>[2x]MISVTDLRPGTKVKMDGGLWECVEYQHQKLGRGGAKVVAKFKNLETGATVE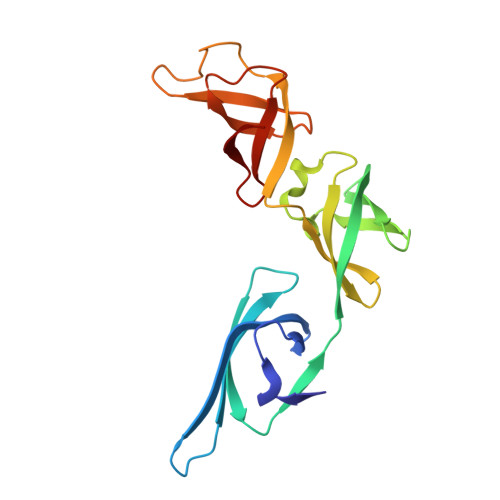RTFNSGEKLEDIYVETRELQYLYPEGEEMVFMDLETYEQFAVPRSRVVGAEFFKEGMTALGDMYEGQPIKVTPPTVVELKVVDTPPGVRGDTVSGGSKPATLETGAVVQVPLFVEPGEVIKVDTRTGEYVGRA(6-but-3-ynyl-4-methyl-5-oxidanyl-pyridin-3-yl)methyl dihydrogen phosphate | 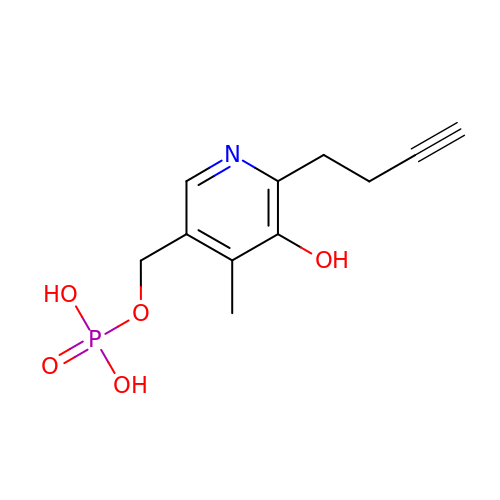C11 H14 N O5 P | HYSIPFHNUDKCJU-UHFFFAOYSA-N>MLAMSPPKPAVELDRHIDLDQAHAVASGGARIVLAPPARDRCRASEARLGAVIREARHVYGLTTGFGPLANRLISGENVRTLQANLVHHLASGVGPVLDWTTARAMVLARLVSIAQGASGASEGTIARLIDLLNSELAPAVPSRGTVGASGDLTPLAHMVLCLQGRGDFLDRDGTRLDGAEGLRRGRLQPLDLSHRDALALVNGTSAMTGIALVNAHACRHLGNWAVALTALLAECLRGRTEAWAAALSDLRPHPGQKDAAARLRARVDGSARVVRHVIAERRLDAGDIGTEPEAGQDAYSLRCAPQVLGAGFDTLAWHDRVLTIELNAVTDNPVFPPDGSVPALHGGNFMGQHVALTSDALATAVTVLAGLAERQIARLTDERLNRGLPPFLHRGPAGLNSGFMGAQVTATALLAEMRATGPASIHSISTNAANQDVVSLGTI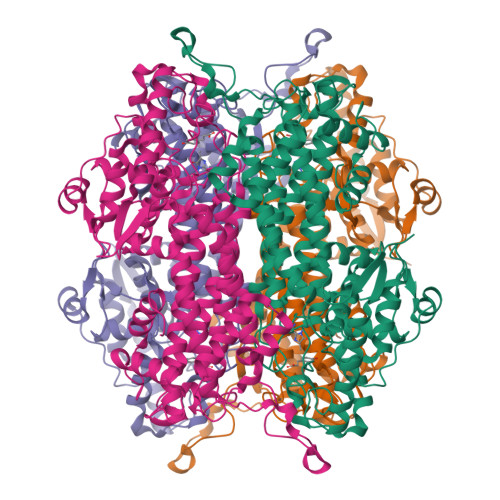AARLCREKIDRWAEILAILALCLAQAAELRCGSGLDGVSPAGKKLVQALREQFPPLETDRPLGQEIAALATHLLQQSPV[8x]> SSQIRQNYSTEVEAAVNRLVNLYLRASYTYLSLGFYFDRDDVALEGVCHFFRELAEEKREGAERLLKMQNQRGGRALFQDLQKPSQDEWGTTLDAMKAAIVLEKSLNQALLDLHALGSAQADPHLCDFLESHF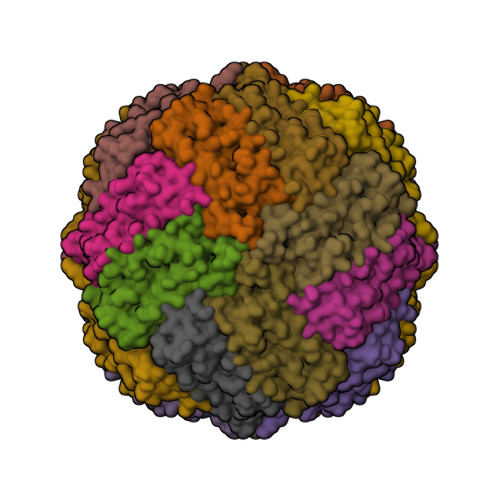LDEEVKLIKKMGDHLTNIQRLVGSQAGLGEYLFERLTLKHD>QYKDNIRHGVCWIYYPDGGSLVGEVNEDGEMTGEKIAYVYPDERTALYGKFIDGEMIEGKLATLMSTEEGRPHFELMPGNSVYHFDKSTSSCISTNALLPDPYESERVYVAESLISSAGEGLFSKVAVGPNTVMSFYNGVRITHQEVDSRDWALNGNTLSLDEETVIDVPEPYNHVSKYCASLGHKANHSFTPNCIYDMFVHPRFGPIKCIRTL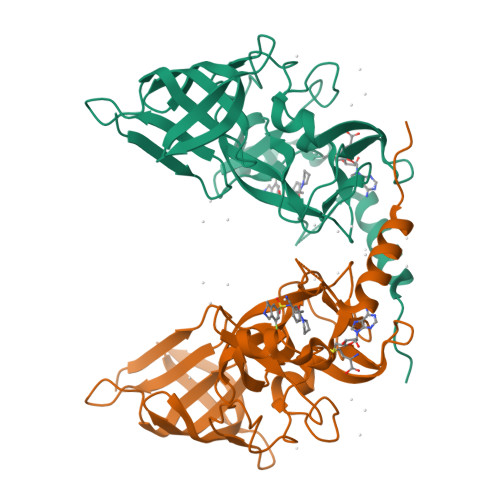RAVEADEELTVAYGYDHSPPGKSGPEAPEWYQVELKAFQATQQKHHHHHH[4x]> VADAHTQGFSLAQYLQEQKTIVETALDQSLVITEPVTIYEAMRYSLLAGGKRLRPILCLAACEMLGGTAAMAMNTACALEMIHTMSLIHDDLPAMDNDDLR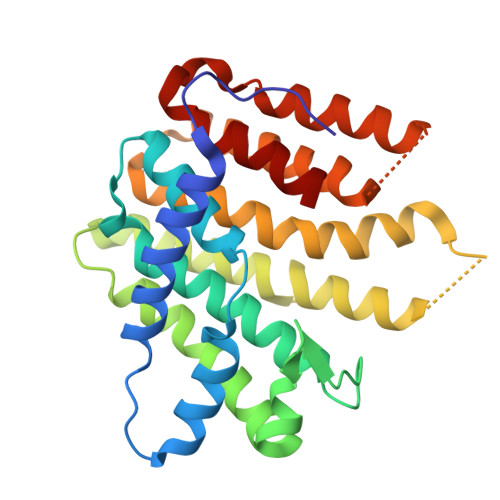RGKPTNHKVYGEDIAILAGDALLSYAFEYVARTPDVPAERLLQVIVRLGQAVGAEGLVGGQVVDLESEVAVETLNFIHTHKTGALLEVCVTAGAILAGAKPEEVQLLSRYAQNIGLAFQIVKSQAEAQKLVAEAIASLEPYGEKANPLKALAEYIVNR>SFMVSLESSRTQYVNQLRSHAQDAATALALSLTPNIDDP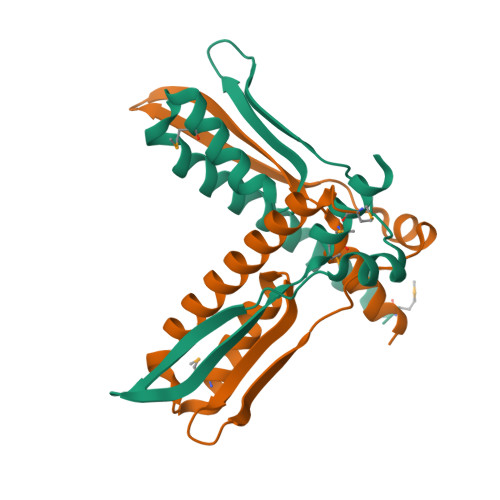AMVELLVSSIFDSGYYSSIRVVDLKTDQTIVERNGIPAVTNVPDWFVKLIGLEPAGGDALVSRGWEQAARVEVVSHPMFALAKLWQSALGS[2x]>AFTGVERSTIGAIAKILASTPEAYGAEALARLFATHPGAKSYFDYADYSAAGAKVQLHGGKVIRAVVSAAEHDDDLHAHLMVLAVTHGKKLLVDPSNFPMLSECILVTLATHLAEFSPATHCAVDKLLSAISSELSSKYR[2x];>[2x]VHWTQEERDEIVKTFFSANSSAIGTKALERMFVVFPWTNAYFAKXXXFSASIHAAIVVGALQDAVKHEDDVKAEFVNISKAHADKLHIDPGSFHLLTDSFIVELAHLKKVAFTPFVFAVWIKFFQVVIDAISSQYH

Haemoglobin (Hb) is a tetrameric iron-containing protein that carries oxygen from the lungs to tissues and carbon dioxide from tissues back to the lungs. The haemoglobin molecule consists of four polypeptide chains, namely two α chains, each with 140 amino acids and two β chains each having 136 amino acids. Distinctly, the SMSs are warm-blooded animals with an advanced circulatory system which is capable of maintaining elevated muscle temperatures up to 33 K above the ambient water temperatures at a depth of 150–500 m with a diverged air-breathing mechanism compared with other vertebrates. The SMS haemoglobin (Hb) structure belongs to the family Lamnidae.

The SMS Hb was found to crystallize in monoclinic space group P21 using the hanging-drop vapour-diffusion method at room temperature. The crystal packing parameters for the SMS Hb structure contain one whole biological molecule in the asymmetric unit with a solvent content of 47%. The sequence identity of SMS Hb compared with human and mustelus griseus shark Hb shares 41 and 80% for the α-chain and 35 and 66% for the β-chain, respectively. In the β chain, three deleted residues (45, 46 and 47) were found in between the C and E helices when compared with the sequence of MGS Hb. All known cartilaginous fish Hb sequences have lost three and four residues between the C and E helices and are thought to lose the D helix in the β chain. The superimposed root-mean-square deviation (RMSD) value between the MGS deoxy T state Hb and SMS Hb is 0.518 Å and between the MGS deoxy and MGS carbonmonoxy Hb is 0.912 Å, revealing a high degree of similarity in the α1β1 dimer. The RMSD value of the non-superimposed α2β2 dimer between SMS Hb and MGS deoxy T state Hb is 2.098 Å, which is smaller when compared with 11.170 Å for the MGS CO form R state. From the quaternary structural features, it is learnt that the SMS Hb and MGS deoxy Hb quaternary structures are similar and adopt an unliganded deoxy T state. The SMS Hb has four hydrogen bonds and 86 non-bonded contacts in the α1β1 interface region and shows the compact nature of the structure. The total iron–iron distance of SMS Hb, 135.35 Å, is comparable with the T state, while in MGS Hb the total iron–iron distance difference is more when compared with other liganded Hbs.3-CHLORO-2,2-DIMETHYL-N-[4-(TRIFLUOROMETHYL)PHENYL]PROPANAMIDE | C12 H13 Cl F3 N O | 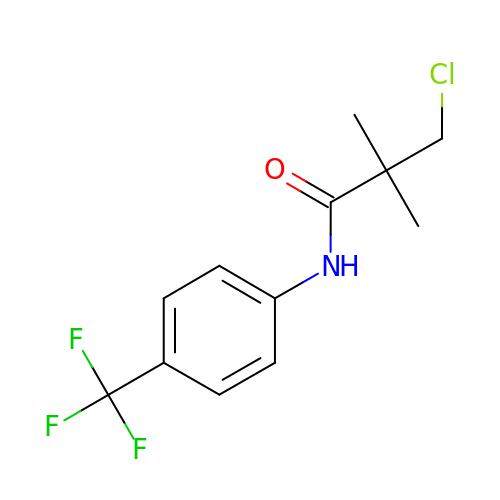QCQZFHOGRCQNIH-UHFFFAOYSA-N>[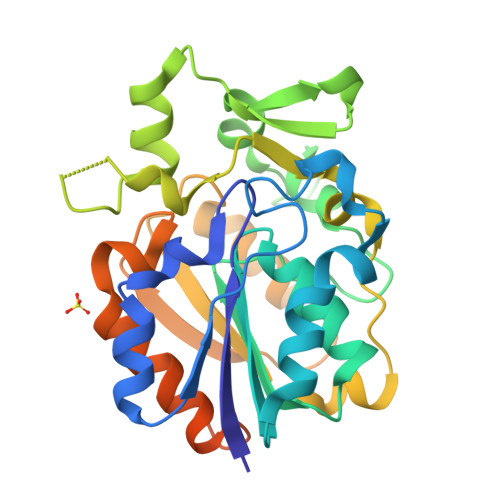6x]MTVTDIILIHGALNRGACYDAVVPLLEARGYRVHAPDLTGHTPGDGGHLSVVDMEHYTRPVADILARAEGQSILLGHALGGASISWLAQHHPDKVAGLIYLTAVLTAPGVTPETFVLPGEPNRGTPHALDLIQPVDEGRGLQADFSRLERLREVFMGDYPGEGMPPAEHFIQTQSTVPFGTPNPMEGRALEIPRLYIEALDDVVLPIAVQRQMQKEFPGPVAVVSLPASHAPYYSMPERLAEAIADFADAPAEYRQTATKAGPDRPAGADGGRADRADLPLEHHHHHH> TDKERFIASLMARMSNAEKIGQLRLVSVGADHPKEALMADIRAGKVGAIFNTVTRPDIRAMQDQVRHSRLKIPLFHAYDVAHGHRTIFP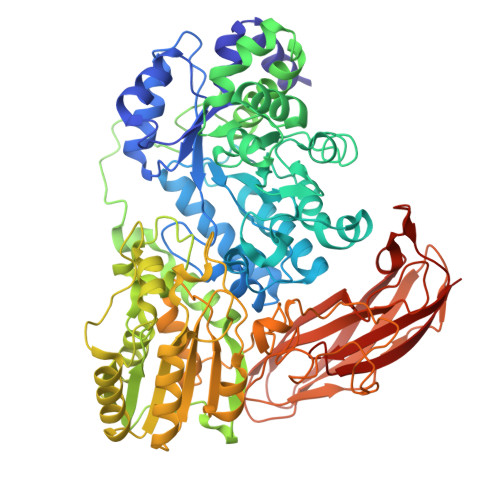ISLGLAASWDPEVVARSARISALEASADGLDMSFSPMVDITRDARWGRVSEGFGEDTYLTSLLSGVMVRAYQGSNLAAPDSIMAAVKHFALYGAAEGGRDYNTVDMSLPRMFQDYLPPYKAAVDAGAGAVMVSLNTINGVPATANRWLLTDLLRQQWGFKGLTISNHGAVKELIKHGLAGNERDATRLAIQAGVDMNMNDDLYSTWLPKLLAAGEIDQADIDRACRDVLAAKYDLGLFADPYRRLGKPDDPPFDTNAESRLHRQAAREVAREGLVLLKNRDGLLPLKKQGRIAVIGPLAKSQRDVIGSWSAAGVPRQAVTVYQGLANAVGERATLLYAKGANVSGDQAILDYLNSYNPEVEVDPRSAEAMLEEALRTARDADLVVAVVGESQGMAHEASSRTDLRIPASQRRLLKALKATGKPLVLVLMNGRPLSLGWEQENADAILETWFSGTEGGNAIADVLFGEHNPSGKLTMSFPRSVGQVPVYYNHLNTGRPMDHDNPGKYTSRYFDEANGPLYPFGYGLSYTEFSLSPLRLSSERLARGATLEARVTLSNSGKRAGATVVQLYLQDPVASLSRPVKELRGFRKVMLEPGESREIVFRLGEADLKFYDSQLRHTAEPGEFKVFVGLDSAQTESRSFTLL> SNAAQQVQQPVAQQQVQQPAQQNTNTA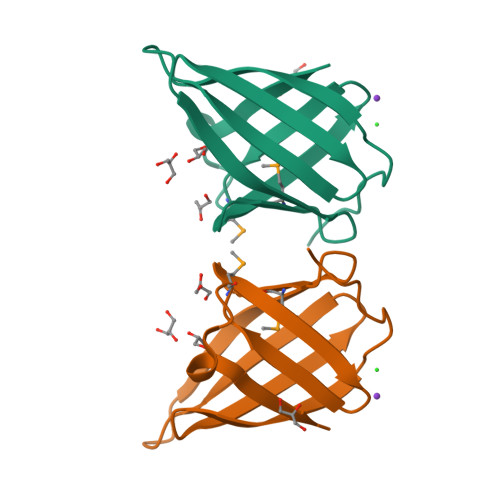NAGGNQNQAAPVQNQPVAQPTDIDGTYTGQDDGDRITLVVTGTTGTWTELESDGDQKVKQVTFDSANQRMIIGDDVKIYTVNGNQIVVDDMDRDPSDQIVLTK>GSMDMEPDVRITNLNLHKGHRVEVRGRIAKGTNRFAVDLGTDSRNLICHCNPRFEYSVDKNTIVLNSKQNDVWDIEKKETAFPFKSGSETMLIFDFEDCITVHLPDGKEIPFTC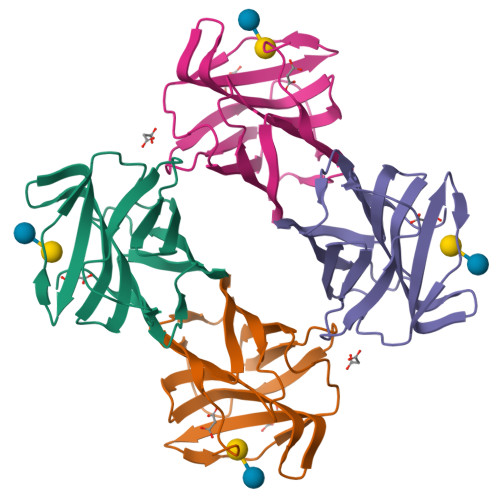RFPIEVINYLALNNIELISISVH[2x]>[2x]STGSAMSQKHLQINQTFEELRLVTQDTENELKKLQQTQEYFIIQYQESLRIQAQFGPLAQLSPQERLSRETALQQKQVSLEAWLQREAQTLQQYRVELAEKHQKTLQLLRKQQTIILDDELIQWKRRQQLAGNGGPPEGSLDVLQSWCEKLAEIIWQNRQQIRRAEHLCQQLPIPGPVEEMLAEV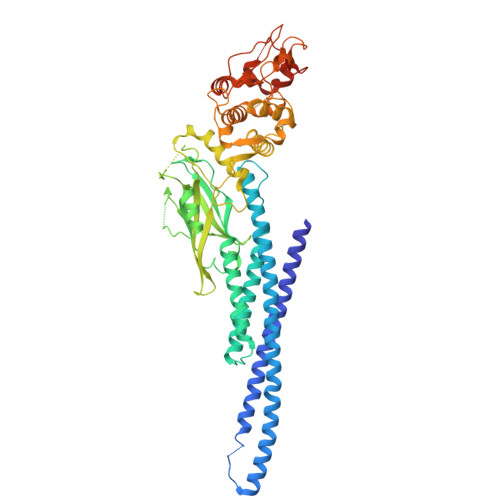NATITDIISALVTSTFIIEKQPPQVLKTQTKFAATVRLLVGGKLNVHMNPPQVKATIISEQQAKSLLKNENTRNDYSGEILNNCCVMEYHQATGTLSAHFRNMSLKRIKRSDRRGAESVTEEKFTILFESQFSVGGNELVFQVKTLSLPVVVIVHGSQDNNATATVLWDNAFAEPGRVPFAVPDKVLWPQLCEALNMKFKAEVQSNRGLTKENLVFLAQKLFNNSSSHLEDYSGLSVSWSQFNRENLPGRNYTFWQWFDGVMEVLKKHLKPHWNDGAILGFVNKQQAHDLLINKPDGTFLLRFSDSEIGGITIAWKFDSQERMFWNLMPFTTRDFSIRSLADRLGDLNYLIYVFPDRPKDEVYSKYYTPVPCESATAKAVDGYVKPQ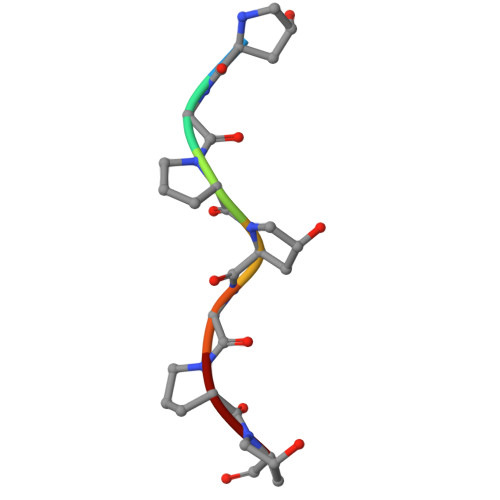> PGPPGPP>CCIGTACCGG[2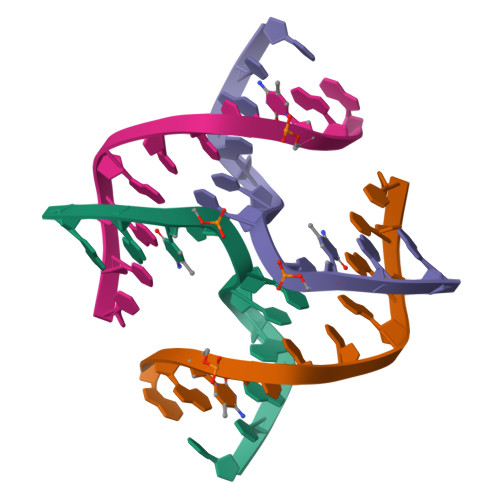x]>[2x]MHHHHHHITSLYKKAGFMSNEYVALITARGGSKGLLRKNVLPLHGIPLIGWTIKAAQGCSYISKVFVSTDDYEIAKISEGLGALVINRPEELATDTASSIDVILHAISWLEQKEVQKYEGMILLQPTSPLRTSHHIKEAIELYEKTAAKFVISVFEPTHTPIKSYLENDDGTISGLYSNEAPYQRRQDLPRAYQPNGAIYAFSIDEFKLNNHFPRNKVFPYVMSEVESADIDTLEDLRKVEEQLKIKEINK

The first step of the incorporation pathway involves the activation of sialic acid to a cytidine monophosphate diester form catalyzed by CMP-sialic acid synthetase (EC 2.7.7.43), a ubiquitous enzyme that is found in both prokaryotes and eukaryotes. In the presence of Mg2+, CMP-sialic acid synthetase (CMAS) catalyzes a sequential ordered reaction that involves a nucleophilic attack on the α-phosphate of CTP by the anomeric O atom of β-Neu5Ac and the production of CMP-sialic acid and pyrophosphate (PPi). The activated sialic acid is then incorporated into LOS or LPS by sialyltransferases. In this report, we present crystal structures of the apo form of the VcCMAS enzyme and of that complexed with cytidine diphos­phate (CDP) and Mg2+.

The final refined apo VcCMAS model contains protein residues 3–226 (subunit A) and 3–228 (subunit B) plus two Ca2+ ions. Residues 13–20 in the phosphate-binding (P) loop and residues 74–79 are disordered in the apo structure. In this study, we have characterized the structural and functional properties of the CMAS enzyme (WP_000064388.1) from V. cholerae. Both the apo and nucleotide-bound structures possess all five of the structural motifs responsible for ligand binding in CMAS enzymes. Several main-chain antiparallel hydrogen-bond interactions between β7 and β10 along with side-chain hydrogen-bond interactions, salt bridges and hydrophobic interactions stabilize the dimerization domain and bury ∼1429 Å2 of each monomer in the dimer interface. In order to identify the dynamics of the domain movement observed upon CDP binding and the residues involved in the hinge-bending motion, we performed DynDom analyses on the apo VcCMAS (conformer I) and CDP–VcCMAS (conformer II) structures. DynDom identified two dynamic domains: the globular domain as the fixed domain (domain 1; residues 1–138 and 179–228) and the extended dimerization domain as a moving domain (domain 2; residues 139–178). Residues 139–142 and 175–178 are identified as the hinge residues. Upon CDP binding, the moving domain bends ∼15–20° around the hinge axis, which results in a partially closed conformation.>[4x]MAKRKIQRYVRKDGKCNVHHGNVRETYRYLTDIFTTLVDLKWRFNLLIFVMVYTVTWLFFGMIWWLIAYIRGDMDHIEDPSWTPCVTNLNGFVSAFLFSIETETTIGYGYRVITDKCPEGIILLLIQSVLGSIVNAFMVGCMFVKISQPKKRAETLVFSTHAVISMRDGKLCLMFRVGDLRNSHIVEASIRAKLIKSKQTSEGEFIPLNQTDINVGYYTGDDRLFLVSPLIISHEINQQSPFWEISKAQLPKEELEIVVILEGMVEATGMTCQARSSYITSEILWGYRFTPVLTLEDGFYEVDYNSFHETYETSTPSLSAKELAELANRAESNSLEVLFQ

All Kir channels are tetramers of identical or related subunits that encode a K+ selectivity filter-containing transmembrane pore (TMD for transmembrane domain) and a cytoplasmic domain (CTD). G-protein-gated inward rectifier K+ (GIRK) channels are activated by both PIP2 and Gβγ. Detailed mechanistic studies in a reconstituted system using a neuronal isoform of GIRK (GIRK2) showed that both PIP2 and Gβγ are required to open the pore. The main conclusion of this study is that GIRK channels – GIRK2 as well as GIRK1/4 – can adopt extended and docked conformations.

In the absence of PIP2 it is clear that GIRK2 can adopt a conformation in which the CTD is disengaged from the TMD and the TMD-CTD linker has to be extended to account for the separation between the TMD and CTD. Thus, in the absence of PIP2, the global conformation of GIRK2 appears much like the Kir2.2 channel in the absence of PIP2 (i.e. both channels adopt an extended conformation) (Tao et al., 2009). Using X-ray crystallography, we had determined a structure of GIRK2 in the absence of PIP2 (CrystalApo) that did not adopt this extended conformation (Whorton and MacKinnon, 2011). The crystal lattice offers a possible explanation for conformational differences between CryoEMApo and CrystalApo. Because in the extended conformation the CTD and TMD are free to move with respect to each other without hindrance, these two structured regions may have been pushed together when the crystal was formed. We think that crystal contacts in the previous CrystalApo structure pushed the CTD and TMD into close proximity. Four classes (1-4) were similar to each other and showed a disengaged CTD (i.e. extended conformation) with an unresolved TMD-CTD linker. The sidechains of positively charged residues that coordinate PIP2 are disordered in the CryoEMApo structure. In the absence of PIP2, the inner helix gate of GIRK2 is most tightly constricted at position Phe192 in the inner helix, which lines the pore on the intracellular side of the selectivity filter.(1S,2S,3R,4S,6R)-3-{[2-(acetylamino)-6-amino-2,3,6-trideoxy-alpha-D-ribo-hexopyranosyl]oxy}-4,6-diamino-2-hydroxycyclohexyl 3-amino-3-deoxy-alpha-D-glucopyranoside 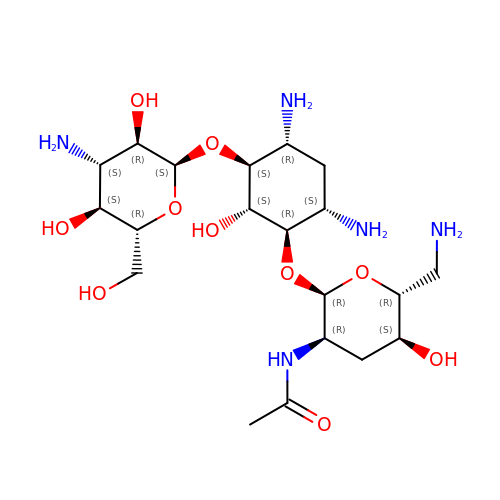| C20 H39 N5 O10 | DMDYSSAQCCMAGB-VMNCQBCKSA-N>DGANSDAAKEYLTKDSFSYEVYGIIAMQAAYRDYDSGDAKQDDNLGGMQLNNESRIGFRGKKQFANFEPTFIWQIEGGYVDPSFGGEGAGLGERDTFVGFESASWGQVRLGRVLTPMYELVDWPASNPGLGDVYDWGGAIGGAKYQDRQSNTIRWDSPMYADKFSIDAAVGAGDKAGLGAGDDYWGGIAAHYKLGPLQLDAAYEGNRNIEAEGQTWENNTYLVGVQGWFENGISFFAQYKYMEADASNGVNEKQDAMSAGLMYTTGDWQYKLGYAANFDLERDGKTLSNTSDDVVSAQIMYFVDPSAVLYARARMNDFNEGLDGLDDAARWTSGTNGDYNEYSVGVEYYF[3x]

The gene encoding for ChiP is found in most marine members of the Vibrionaceae, emphasizing the general importance of this OM diffusion channel for chitin utilization. The addition of micromolar concentrations of chitooligosaccharides such as chitohexaose (GlcNAc6) causes a complete block of ionic current, demonstrating tight binding. Here, we report X-ray crystal structures of VhChiP in the absence and presence of chitooligosaccharides.

Given that the channels of the OM-expressed apo-protein are closed due to the insertion of the N-terminus of a neighboring monomer, it is important to establish whether the incoming substrate from the extracellular space could displace the N-terminus to bind in the pore. To answer these questions we co-crystallized OM-expressed VhChiP with chitotetraose (GlcNAc4). OM-expressed VhChiP in the presence of the GlcNAc4 substrate also crystallizes under the same conditions and in the same space group as the closed apo-protein. Importantly, the oligosaccharide is bound in the channel and has displaced the N-terminus, which is now in the periplasmic space and has the same conformation as that of the in vitro-folded protein. The GlcNAc4 substrate occupies approximately the positions of GlcNAc-2 to GlcNAc-5 of the GlcNAc6 chain, suggesting that the central positions of the binding site provide the most binding energy for chitooligosaccharides (note that the subunits of GlcNAc4 are numbered 2–5 to provide consistency with those of chitohexaose). However, there are differences of up to 5 Å for individual atoms between the two structures, especially at both ends of the substrate (GlcNAc-2 and GlcNAc-5). In most cases, however, this does not dramatically change the interactions between the sugar and the channel. For example, the acetamido carbonyl group GlcNAc-2 interacts in both structures with Asn127 and Arg312 whereas that of GlcNAc-3 interacts with Arg94/148. It appears therefore that VhChiP accommodates compounds of different length via subtle changes in the way the substrates are bound. For compounds of four GlcNAc units or larger, the central binding sites (2–5) are likely to be always occupied, in a manner as observed in our structures.> VEPSGHAADRIARLPGQPAVDFDMYSGYITVDEGAGRSLFYLLQEAPEDAQPAPLVLWLNGGPGCSSVAYGASEELGAFRVKPAGAGLVLNEYRWNKVANVLFLDSPAGVGFSYTNTSSDIYTSGDNRTAHDSYAFLAKWFERFPHYKYRDFYIAGESYAGHYVPELSQLVHRSKNPVINLKGFMVGNGLIDDYHDYVGTFE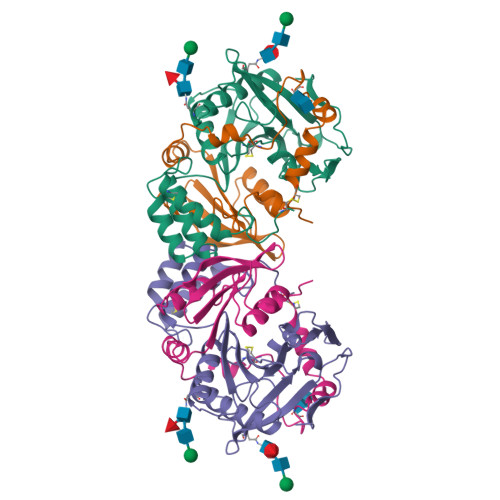FWWNHGIVSDDTYRRLKEACLHDSFIHPSPACDAATDVATAEQGNIDMYSLYTPVCN;> SYDPCTERYSTAYYNRRDVQMALHANVTGAMNYTWATCSDTINTHWHDAPRSMLPIYRELIAAGLRIWVFSGDTDAVVPLTATRYSIGALGLPTTTSWYPWYDDQEVGGWSQVYKGLTLVSVRGAGHEVPLHRPRQALVLFQYFLQGKPMPG>[2x]MASSHHHHHHHENLYFQGMTDTEVAQITDNPYKADFPILAANPKVAYLDSAATSQRPRVVIEAQSRFYETMNANALRGLYRWSVDATAAIEDARASIAKFIGAVDKNDKPESQQIIFTRN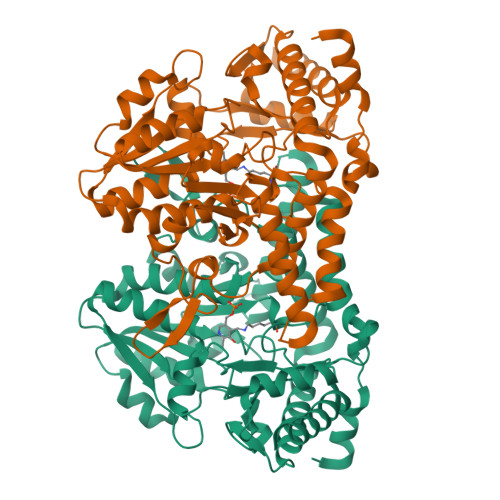TSEALNLVASSLGRYALKPGDDVVISIMEHHSNIIPWQQICKATGANLVYLRMNSQYQITPEEIASKITERAKIVSVTHVSNVLGTRNDIKAIAKRTHAMGAYMVVDAAQSAPHILVNVHDLDCDLLAFSAHKMCGPMGIGVLWGRAELLNAMPPFLTGGEMIDSVTETGAVWAPVPEKFEAGTQDAAGIYATGAAIKYLNGLDMAKIEKREELLARYLVQQLCTLDFVDIVGSKLGQNHVGAVAFNVRGVHPHDVSSILDMNNVCIRAGHHSAEPLLIELHESSTCRASVAFYNDKHDIDQLIEGLNQVWKIFGSAVNTKQNKELK>GSSGSSGMPMTLGYWDIRGLAHAIRLFLEYTDSSYEEKRYTMGDAPDYDQSQWLNEKFKLGLDFPNLPYLIDGSHKITQSNAILRYLGRKHNLCGETEEERIRVDILENQLMDNRMVLARLCYNADFEKLKPGYLEQLPGMMRLYSEFLGKRPWFAGDKITFVDFIAYDVLERNQVFEAKCLDAFPNLKDFIARFEGLKKISDYMK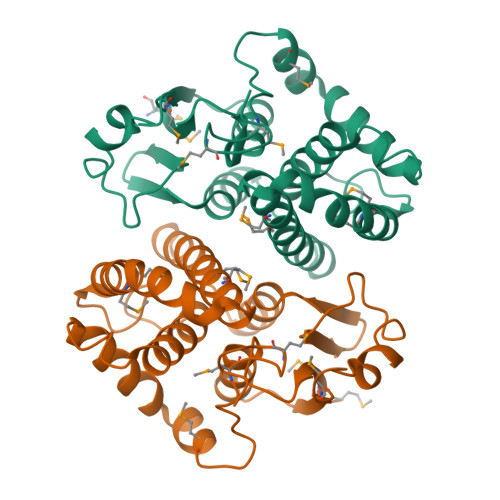TSRFLPRPMFTKMATWGSNSGPSSG[2x]> GGGTTAGGGTTAGGGTTTGGG

The DNA G-quadruplex is known for forming a range of topologies and for the observed lability of the assembly, consistent with its transient formation in live cells. Single-stranded DNA is found naturally at the ends of chromosomes, which in humans consists of several hundred repeats of the telomeric base sequence (T2AG3)n.2−5 In this case, a specific structure composed of guanosine residues, the G-quadruplex or G4, can form in the presence of K+ ions, which are naturally present at ∼100 mM concentrations in human cells. The resulting assembly is known from X-ray6 and nuclear magnetic resonance (NMR)4 studies to give a range of folds of the DNA backbone, held together by the central K+ ions and made possible by the rotation of the guanine base relative to its attached sugar. The stabilization of a particular topology by a small molecule is of great importance for therapeutic applications.

Here, we show that the ruthenium complex Λ-[Ru(phen)2(qdppz)]2+ displays enantiospecific G-quadruplex binding. It crystallized in 1:1 stoichiometry with a modified human telomeric G-quadruplex sequence, GGGTTAGGGTTAGGGTTTGGG (htel21T18), in an antiparallel chair topology, the first structurally characterized example of ligand binding to this topology. The bound ruthenium complex is notable for its asymmetrically fused anthraquinone-dppz chromophore and its lambda chirality. The extended ligand of the ruthenium complex is bound at one end of the G4 stack in the narrow second lateral loop, and can be thought of as intercalated between a T10–A12 Hoogsteen base pair and the adjacent G-quartet, as shown in Figure 3b,c. In this case, the syn nucleosides are G13 and G1, with G13 the nucleoside determining the enantiomeric specificity and the base orientation, with a contact between the G13 ribose sugar and the adjacent phen ring of the ligand. The chromophore overlaps with all the four bases of the quartet and shows an unexpected curvature that matches the deviations from planarity in the flanking G-quartet. A key difference between the anticlockwise and clockwise structures is that in the arrangement seen here, the first and third loops bridge the wide grooves of the structure, with the second loop, where the complex is bound, bridging a narrow groove. One advantage of an X-ray structure determination is that the cation assembly holding the G-quartets can be unambiguously determined, with three fully occupied K+ ion positions clearly visible in the center of the G-quadruplex assembly, confirming a clear preference for K+. The third K+ coordinates three thymine carbonyl groups (T5, T16, and the deliberately introduced variant T18) with the eighth coordination position occupied by a water molecule.> TRPNHTIYINNLNSKIKKDELKKSLH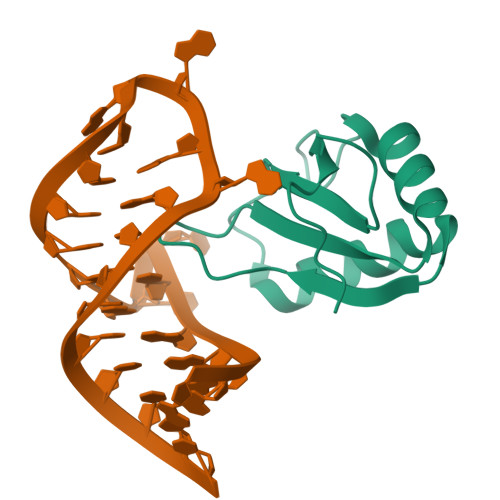AIFSRFGQILDILVPRTRRPRGQAFVIFKEVSSATNALRSMQGFPFYDKPMAIQYAKTDRTI> MATGRIQFAVSTPCNTKGKPSGYRLFEFKNDRLALVPSERGCTKVDVNANIQAFCYLRPNGRDTSISPDATHILDSCDYMVLAKSNGFIEIISNYQYKIKNGLRLAPSYILRCTPEDFESNFFSDYMIAGLEYSQGLLYCCMCSGRIYVFVMNLPTDYIQYKNMYNPMFPDCFFKVHHDNNTTHSSEEEKLFEGSTRYTGRSCSKHICYFLLPIEPSHLRSSPVVSSFCNMYQGLPIYRPSMYLHIERGISTFHINPLDRFCFMTVSPRSPLF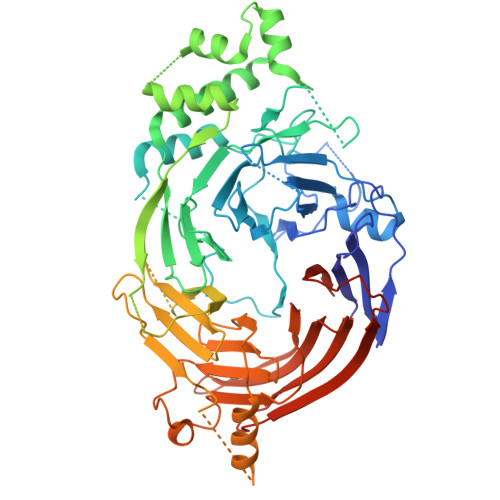IRKIILPLTYVTFLSTFISLKNSIQGDTCGEILSWDNVAQQNGFGSLFSWISNKFTFDTDIINSTIWDDIVKYSGTGMLDSGIVWKQRQGHAKDDIYELFHTQDMLGSSRRNSSFSTASSEPRPLSRRRRESFQALTRDAFRERMDVPCSTKWELDSFIRGLRRNTFMVDFEIVEKISHRNGNDGVNEDDNTTDESDETMTSFLTDNYKKMDIVCIDHFVTLSAFRPRYYDEPIIKIDSLSNKNGSENGTNEEEWAESQMKVDGQVIDDETAQFKQALGNLCSFKKLFMLDDSLCFILDTHGVLLINRFEIKNTKNLLRNSKDTIRIIPHDFGLINDTIVIINDIDVGTDNVCALTFHLVVTSMAGEITVLKGEFFKNCRLGRIKLCDSLKLNRKDRFVDKLALIDYDGLNAQKRRLDYDEKDLYTFIVKKVKRD>[4x]MAHHHHHHSSGLEVLFQGPMTRTVSVLSAASALPGPTVDNATLGRRLGMDRLWEQWVDAFIGTRTRHLAVDLDSGEIRHTLADLAHQAGSRALDAAGVTPEEVDLVVLGTATPDRLMPTTATVVADRLGIDGVPAYQLQSGCSGAVQALAVTRSLLLGGTARTALVLGGDVVARFYDLTADLRKLPPAEFVNYVLFGDGVGAAVLRVGEVAGAAALRSVFTRLVGLGREPGATLEWFGPTEDRNRPA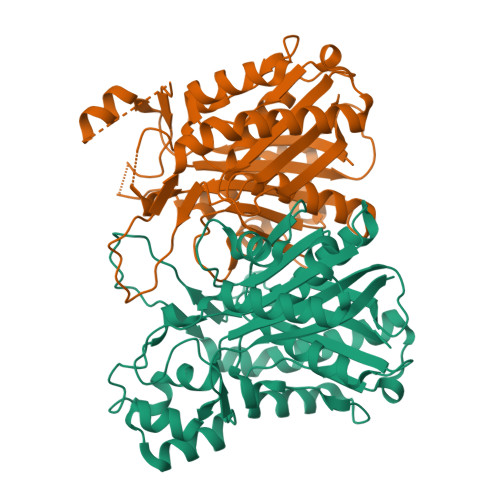ATEDYKAIERHVPDLAAEVVEELLGELGWARDDLDYVLPPQLSGRMTALIVERLKLPQATEVSCVAETGNNGNGIVFLQLERALARLAGGQRALGVSIESSKWIKSGFALEGL>[6x]MLCVDVNVLVYAHRADLREHADYRGLLERLANDDEPLGLPDSVLAGFIRVVTNRRVFTEPTSPQDAWQAVDALLAAPAAMRLRPGERHWMAFRQLASDVDANG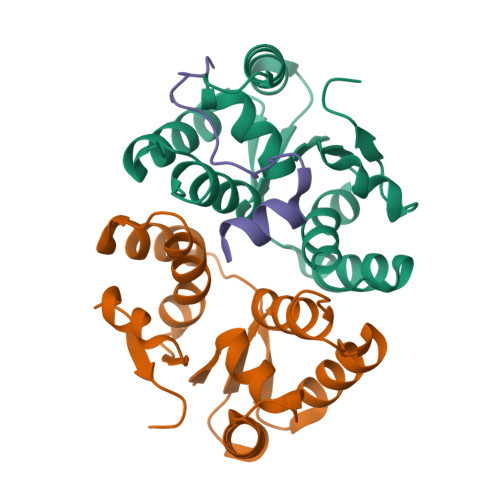NDIADAHLAAYALENNATWLSADRGFARFRRLRWRHPLD;>[3x]YRVQPSGKGGLRPGVDLSSNAALAEAMN>MSLKITEVKAHALSTPIPERMRVESGAGLKLNRQMILVEVRTDEGVTGVGSPSGPYDLAVLKRAIEDVIGPQLIGEDPANINYLWHKVFHGEVSRNLGHRSVGIAAMSGVDIALWDLKGRAMNQPIYQLLGGKFHTRGVRAYASSIYWDLTPDQAADELAGWVEQGFTAAKLKVGRAPRKDAANLRAMRQRVGADVEILVDANQSLGRHDALAMLRILDEAGCYWFEEPLSIDDIEGHRILRAQGTPVRIATGENLYTRNAFNDYIRNDAIDVLQADASRAGGITEALAISASAASAHLAWNPHTFNDIITVAANLHLVAASPHPAMFEWDITHNDLMTRLASYDLKLENGLVQPPQGPGLGFEIDWDFVAAHAWKGEP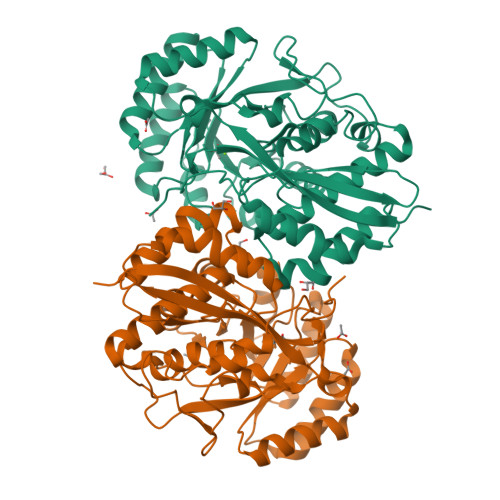AIGAGHGMKK[2x]>[2x]GHMKDLKGTKTAENLKQGFIGESMANRRYLYFAK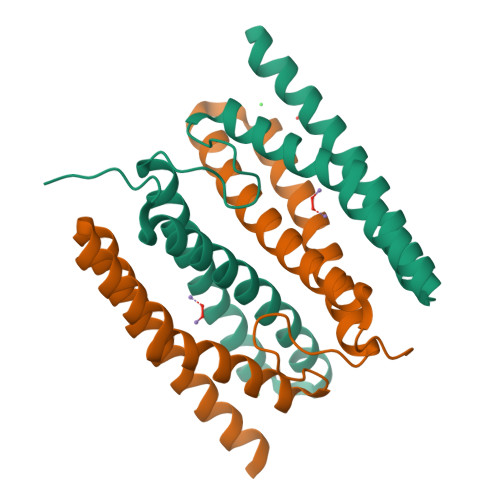RADEEGYPEIAGLLRSIAEGETAHAFGHLDFIRQGGLTDPATDKPIGTLEQMIESAIAGETYEWTQMYPGFAKVAREEGFPEVAEWFETLARAEKSHAEKFQNVLKQLKGGT> MSAPTDDTPTDAIAAPRHSAPPRPRLPWFLRTFAVPIILAWVAVVAILNTVVPTLDEVGEMRAVSMAPNDAPSTLAIKRVGQVFEEYDTSSSVMIVLEGEEPLGIEAHAFYDKMVADLRADTEHVQHVQDFWGDTLTASGAQSVDGKAAYVQVYIAGDQGESLANESVEAVRKIATERETPSGVKAYVTGAAATSADQRAEGDASMKLIEGVTFAVITVMLLAVYRSVITTLIVLAMVVLGLSGARGIVAFLGFYNVFGLTTFATNMVVTLAIAAATDYAIFLIGRYQEARRAGEDRESAYYTMFHGTAHVVLASGLTIAGATLCLHFTRLPYFQTMGVPLAIGMLIVVAAALTAGPAVISVVSRFGKTLEPKRFSRSPGWHRVGTATVRWPGAILVCAVVAALIGLLALPGYYTTYDDRRYLPDDVPANVGYDAAFRHFSQAKMNPDLMMVETDRDLRNPADFLVIDKIAKALKNVHGIAQVQTITRPDGDPIEHSTIPYTIGQSGTTQIMNNDYMQTNLDNLLKQADDLQTSIDSMTEMMNIQTELAAVSQSMADKMAQTSDDTADVRDHLADFDDFFRPIRNYLYWEPHCYDIPMCWSMRSIFESIDGINTMSDDFQELVPEMRRMADLMPRMVAVMPAQIQSMKNQKQTLLNQYQVQKAQQDQNMAMQENATAMSQAFDAAKNDDSFYLPPEAFETDDFQRGMKLFMSPDGHAVRFTIIHQGDPLTEEGTARMDELKVAAADAIKGTPFEGARIYLGGSAATYNDMQIGADYDLIIVAASALILIFIIMMVLTRAVVAAAVIVGTVVLSLASAFGLSVLLWQHIVGIPLHWMVLPMSVIVLLAVGADYNLLLVSRMKEEIHAGIRTGIIRAMVGTGAVVTAAGLVFAFTMASMAVSSLITIGQVGTTIGLGLLFDTLVVRSLMTPSIATLLGRWFWWPQRVRERPVPSKWPTPIQRTPEEALS;> MAATQEEIIAGLAEIIEEVTGIEPSEVTPEKSFVDDLDIDSLSMVEIAVQTEDKYGVKIPDEDLAGLRTVGDVVAYIQKLEEENPEAAAALREKFAADQ

The genome of Mtb encodes 13 mycobacterial membrane protein large (MmpL) transporters. These membrane proteins belong to a subfamily of the resistance-nodulation cell division (RND) superfamily of transporters and are critical for mycobacterial physiology and pathogenesis, with several of these transporters involved in the export of fatty acids and lipid components to the cell envelope. MmpL4 and MmpL5 share similar functions in siderophore export and are required for iron acquisition. Mycobacteria secrete mycobactin (Mbt) and carboxymycobactin (Cmb), siderophores with an extremely high affinity for Fe(III), via the MmpL4 and MmpL5 transporters to recruit this important metal that is essential for growth and survival. According to the protein sequence alignment with MmpL3, it is speculated that both MmpL4 and MmpL5 are proton motive force (PMF)-dependent transporters that function via a proton/substrate antiport mechanism.

However, only MmpL5 appears to confer increased resistance to bedaquiline, an FDA approved anti-TB drug. Within the transmembrane domain of the MmpL5 transporter, the conserved residues that make up the proton-relay network are also residues D278, Y279, D851, and Y852.6-azanyl-9-[(2R,3R,4S,5R)-5-(hydroxymethyl)-3,4-bis(oxidanyl)oxolan-2-yl]-1H-purin-2-one 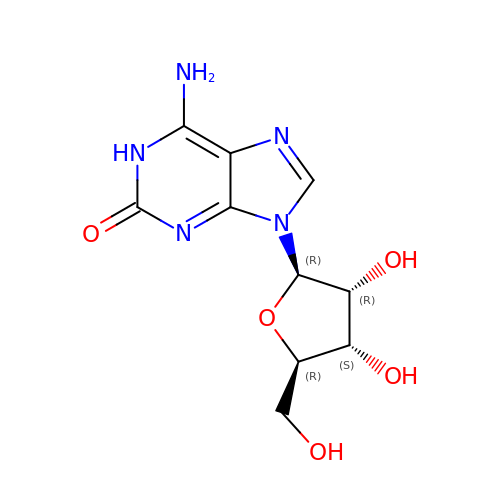| C10 H13 N5 O5 | MIKUYHXYGGJMLM-UUOKFMHZSA-N> MTFAKIKFSAQIRLETGLHIGGSDAFAAIGAINSPVIKDPITNLPIIPGSSLKGKMRTLLAKVYNEKVAEKPSDDSDILSRLFGNSKDKRFKMGRLIFRDAFL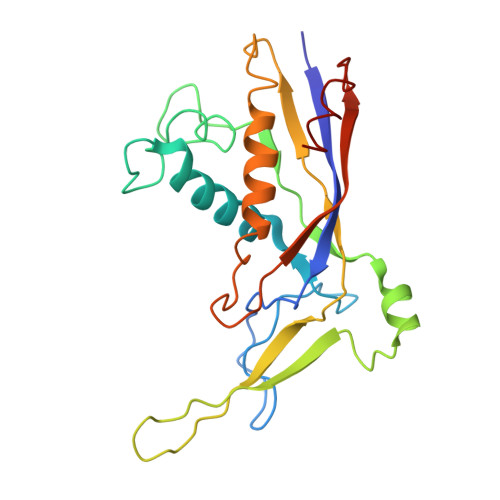SNADELDSLGVRSYTEVKFENTIDRITAEANPRQIERAIRNSTFDFELIYEITDENENQVEEDFKVIRDGLKLLELDYLGGSGSRGYGKVAFENLKATTVFGNYDVKTLNELLTAEV>MTSIQQRDAQSVLAAIDNLLPEIRDRAQATEDLRRLPDETVKALDDVGFFTLLQPQQWGGLQCDPALFFEATRRLASVCGSTGWVSSIVGVHNWHLALFDQRAQEEVWGEDPSTRISSSYAPMGAGVVVDGGYLVNGSWNWSSGCDHASWTFVGGPVIKDGRPVDFGSFLIPRSEYEIKDVWYVVGLRGTGSNTLVVKDVFVPRHRFLSYKAMNDHTA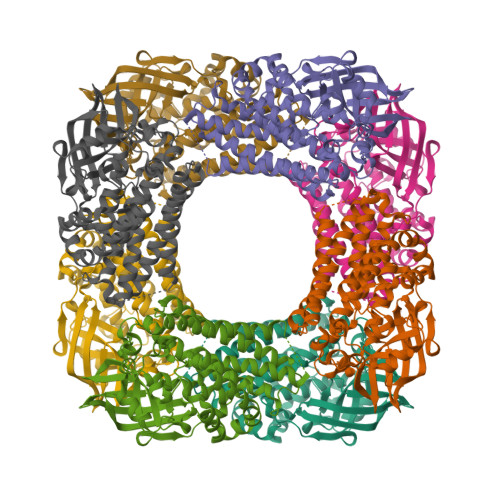GGLATNSAPVYKMPWGTMHPTTISAPIVGMAYGAYAAHVEHQGKRVRAAFAGEKAKDDPFAKVRIAEAASDIDAAWRQLIGNVSDEYALLAAGKEIPFELRARARRDQVRATGRSIASIDRLFEASGATALSNEAPIQRFWRDAHAGRVHAANDPERAYVIFGNHEFGLPPGDTMV[2x]> MSQPQSSQVTKRGLTDPERAAIIAAAVPDHALDTQRKYHYFIQPRWKRLSEYEQLSCYAQPNPDWIAGGLDWGDWTQKFHGGRPSWGNESTELRTTDWYRHRDPARRWHHPYVKDKSEEARYTQRFLAAYSSEGSIRTIDPYWRDEILNKYFGALLYSEYGLFNAHSSVGRDCLSDTIRQTAVFAALDKVDNAQMIQMERLFIAKLVPGFDASTDVPKKIWTTDPIYSGARATVQEIWQGVQDWNEILWAGHAVYDATFGQFARREFFQRLATVYGDTLTPFFTAQSQTYFQTTRGAIDDLFVYCLANDSEFGAHNRTFLNAWTEHYLASSVAALKDFVGLYAKVEKVAGATDRAGVSEALQRVFGDWKIDYADKIGFRVDVDQKVDAVLAGYKN;> MAISLATKAATDALKVNRAPVGVEPQEVHKWLQSFNWDFKENRTKYPTKYHMANETKEQFKVIAKEYARMEAAKDERQFGTLLDGLTRLGAGNKVHPRWGETMKVISNFLEVGEYNAIAASAMLWDSATAAEQKNGYLAQVLDEIRHTHQCAFINHYYSKHYHDPAGHNDARRTRAIGPLWKGMKRVFADGFISGDAVECSVNLQLVGEACFTNPLIVAVTEWASANGDEITPTVFLSVETDELRHMANGYQTVVSIANDPASAKFLNTDLNNAFWTQQKYFTPVLGYLFEYGSKFKVEPWVKTWNRWVYEDWGGIWIGRLGKYGVESPASLRDAKRDAYWAHHDLALAAYAMWPLGFARLALPDEEDQAWFEANYPGWADHYGKIFNEWKKLGYEDPKSGFIPYQWLLANGHDVYIDRVSQVPFIPSLAKGTGSLRVHEFNGKKHSLTDDWGERQWLIEPERYECHNVFEQYEGRELSEVIAEGHGVRSDGKTLIAQPHTRGDNLWTLEDIKRAGCVFPDPLAKF;> MAKREPIHDNSIRTEWEAKIAKLTSVDQATKFIQDFRLAYTSPFRKSYDIDVDYQYIERKIEEKLSVLKTEKLPVADLITKATTGEDAAAVEATWIAKIKAAKSKYEAERIHIEFRQLYKPPVLPVNVFLRTDAALGTVLMEIRNTDY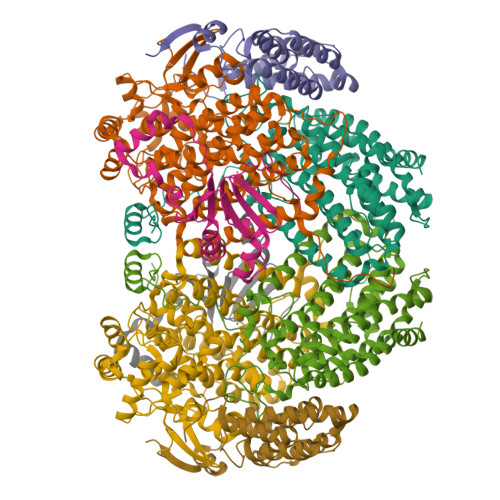YGTPLEGLRKERGVKVLHLQA;> MSSAHNAYNAGIMQKTGKAFADEFFAEENQVVHESNAVVLVLMKSDEIDAIIEDIVLKGGKAKNPSIVVEDKAGFWWIKADGAIEIDAAEAGELLGKPFSVYDLLINVSSTVGRAYTLGTKFTITSELMGLDRALTDI> MPSSLLGAAMPASTSAAALQEALENAGRLIDRQLQEDRMYPDLSELLMVSAPNNPTVSGMSDMDYPLQGPGLLSVPNLPEISSIRRVPLPPELVEQFGHMQCNCMMGVFPPISRAWLTIDSDIFMWNYEDGGDLAYFDGLSETILAVGLVKPKAGIFQPHVRHLLVLATPVDIVILGLSYANLQTGSGVLNDSLSGGMQLLPDPLYSLPTDNTYLLTITSTDNGRIFLAGKDGCLYEVAYQAEAGWFSQRCRKINHSKSSLSFLVPSLLQFTFSEDDPILQIAIDNSRNILYTRSEKGVIQVYDLGQDGQGMSRVASVSQNAIVSAAGNIARTIDRSVFKPIVQIAVIENSESLDCQLLAVTHAGVRLYFSTCPFRQPLARPNTLTLVHVRLPPGFSASSTVEKPSKVHRALYSKGILLMAASENEDNDILWCVNHDTFPFQKPMMETQMTAGVDGHSWALSAIDELKVDKIITPLNKDHIPITDSPVVVQQHMLPPKKFVLLSAQGSLMFHKLRPVDQLRHLLVSNVGGDGEEIERFFKLHQEDQACATCLILACSTAACDREVSAWATRAFFRYGGEAQMRFPTTLPPPSNVGPILGSPVYSSSPVPSGSPYPNPSFLGTPSHGIQPPAMSTPVCALGNPATQATNMSCVTGPEIVYSGKHNGICIYFSRIMGNIWDASLVVERIFKSGNREITAIESSVPCQLLESVLQELKGLQEFLDRNSQFAGGPLGNPNTTAKVQQRLIGFMRPENGNPQQMQQELQRKFHEAQLSEKISLQAIQQLVRKSYQALALWKLLCEHQFTIIVAELQKELQEQLKITTFKDLVIRDKELTGALIASLINCYIRDNAAVDGISLHLQDICPLLYSTDDAICSKANELLQRSRQVQNKTEKERMLRESLKEYQKISNQVDLSNVCAQYRQVRFYEGVVELSLTAAEKKDPQGLGLHFYKHGEPEEDIVGLQAFQERLNSYKCITDTLQELVNQSKAAPQSPSVPKKPGPPVLSSDPNMLSNEEAGHHFEQMLKLSQRSKDELFSIALYNWLIQVDLADKLLQVASPFLEPHLVRMAKVDQNRVRYMDLLWRYYEKNRSFSNAARVLSRLADMHSTEISLQQRLE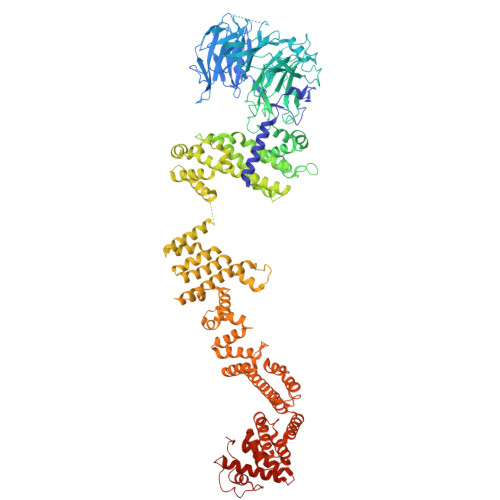YIARAILSAKSSTAISSIAADGEFLHELEEKMEVARIQLQIQETLQRQYSHHSSVQDAVSQLDSELMDITKLYGEFADPFKLAECKLAIIHCAGYSDPILVQTLWQDIIEKELSDSVTLSSSDRMHALSLKIVLLGKIYAGTPRFFPLDFIVQFLEQQVCTLNWDVGFVIQTMNEIGVPLPRLLEVYDQLFKSRDPFWNRMKKPLHLLDCIHVLLIRYVENPSQVLNCERRRFTNLCLDAVCGYLVELQSMSSSVAVQAITGNFKSLQAKLERLH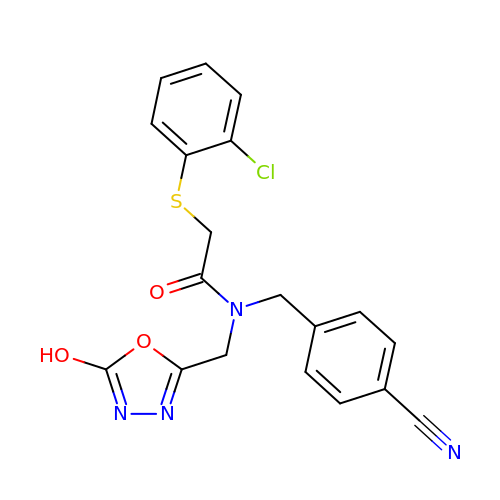2-(2-chlorophenyl)sulfanyl-~{N}-[(4-cyanophenyl)methyl]-~{N}-[(5-oxidanyl-1,3,4-oxadiazol-2-yl)methyl]ethanamide | C19 H15 Cl N4 O3 S | NBNRDDVQRANCKW-UHFFFAOYSA-N The acyl-ACP synthetase (termed AasS) of the zoonotic pathogen Vibrio harveyi recycles exogenous fatty acid (eFA), bypassing the requirement of type II fatty acid synthesis (FAS II), a druggable pathway. Very recently, the AasS (533 aa) of V. harveyi was found to feature a large domain at N-terminus (termed AasS_N) that is connected with a compact C-terminal domain by a flexible linker. As expected, a hexamer ring-like overall structure was invariantly formed in all the three types of AasS particles, regardless of a cofactor/inhibitor. Obviously, the pattern of AasS oligomerization is recognized as a trimer of dimers, which mainly relies on two interfaces constituted by the AasS_N domain.

In addition to the two controls we introduced, (i) AasS alone and (ii) its complex with C10-AMP adenylate, we focused on the complex of AasS liganded with C10-AMS inhibitor. Unlike the two controls that are characterized with a dimension of ‘140x150x80 Å’, the inhibitor-bound AasS architecture is relatively compact, because that its dimension is only confined to ‘130x140x65 Å’. Except for a sulfamoyl moiety that replaces a phosphate group, the C10-AMS inhibitor resembles the C10-AMP intermediate. Structural alignment of C10-AMP adenylate-bound conformation with its C10-AMS inhibitor-liganded form, elucidated that conformational transition is due to the 140° rotation of the compact AasS_C domain. As predicted, C10-AMS inhibitor was also found to bind an array of almost-identical active sites in the AasS_N part. However, AasS_C domain adopts a closed conformation rather than an open state to benefit its C10-AMS recognition. In place of K522 exploited in C10-AMP binding, the AasS_C K432 residue produces several interactions with surrounding oxygen atoms. Additionally, The W437 residue here forms a hydrogen bond with the bridging oxygen atom. Unexpectedly, this inhibitor was found to trap AasS enzyme in a ‘closed’ conformation, which likely represents the enzyme at the very beginning of the second step reaction where the adenylate serves as a substrate, before the binding of the ACP thiol substrate. The resultant blockade prevents other substrates from binding/entering AasS enzyme.

>[6x]MNQYVNDPSNYQLLIKNLLFSPVAFNPEQEIVYANHRRHSYKTFHDRVRQFANALTKMGVKKGDTVAVMDYDSHRYLECYFAIPMIGAKLHMINVRLSPEQILYTIDHAEDDIILIHEEFLPILDQIKGRIDTVTRYVVLRDDEECEYERLLEQESTEYNFPDFDENTVATTFYTTGTTGFPKGVFFTHRQLVLHTMGILSTIGTNASQGRLHQGDIYMPITPMFHVHAWGLPYMATMLGVKQVYPGKYVPDVLLNLIEQEKVTFSHCVPTILHLLLSSPKSKAMDFSGWKVVIGGAALPKALCKSALERDIDVFAGYGMSETGPILSIVQLTPEQLELDVDQQAEYRSKTGKKVALVEAYIVDEDMNKLPHDGETAGEIVVRAPWLTPNYYKDNKNSKALWRGGYLHTGDVAHIDDEGFIKITDRVKDMIKISGEWVSSLELEDILHQHQSVSEVAVIGMPHNKWGEVPLALVTLKEDAQVTEKELLGFAKDFINKGILAREALLLKVKIVDEIAKTSVGKVDKKELRKLH>MRGSHHHHHHGMASMIVVFVGTAGSGKTTLTGEFGRYLEDNYKVAYVNLDTGVKELPYEPSIDVREFVTVEEIMREGYGPNGAIVESYDRLMEKFNEYLNKILRLEKENDYVLIDTPGQMETFLFHEFGVRLMENLPYPLVVYISDPEILKKPNDYCFVRFFALLIDLRLGATTIPALNKVDLLSEEEKERHRKYFEDIDYLTARLKLDPSMQGLMAYKMCSMMTEVLP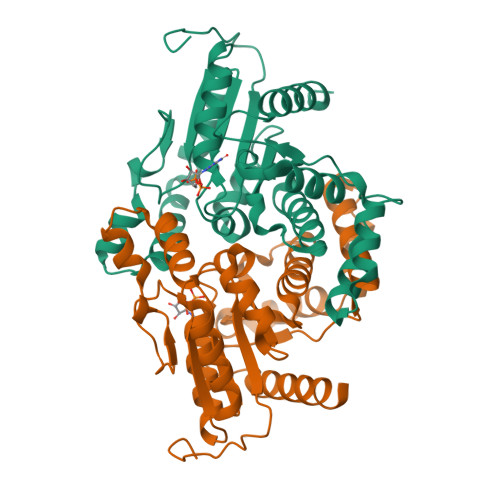PVRVLYLSAKTREGFEDLETLAYEHYCTCGDLT[2x]>GHMVSLTLQVENDLKHQLSIGALKPGARLITKNLAEQLGMSITPVREALLRLVSVNALSVAPAQAFTVPEVGKRQLDEINRIRYELELMAVALAVENLTPQDLAELQELLEKLQQAQEKGDMEQIINVNRLFRLAIYHRSNMPILCEMIEQLWVRMGPGLHYLYEAINPAELR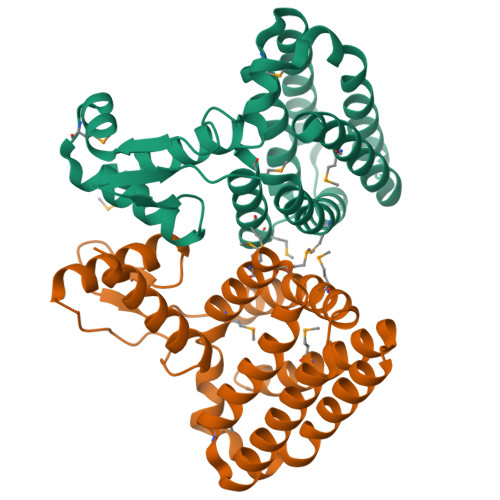EHIENYHLLLAALKAKDKEGCRHCLAEIMQQNIAILYQQYNR[2x]>MVEPGRYRVINVKGGTALDLDINNNSTVHGWAFHGGD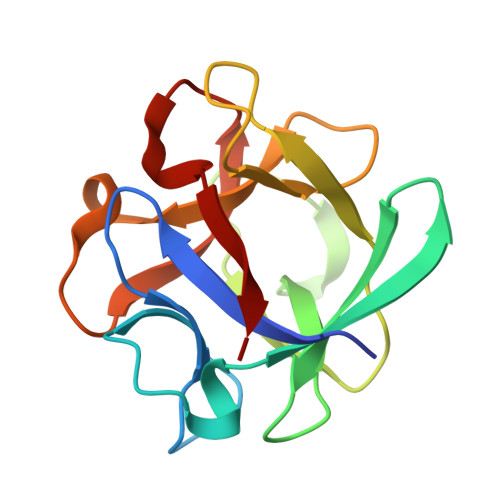NQLWDFEHIGDNIWTICNANTGGYLAIVNGIAGDGVKAVSWADPFEWAVWPDENDGSVWRIGVPDTAFHLDLSDHGNSADGTAVQVWNASDGRNQCWVVEEA[2x]>MGSTGNAEIQIIPTHSSDEEANLFAHQLARAASLPMALKAAIELDVLEIMAKSVPPSGYISPAEIAAQLPTTNPEAPVMLDRVLRLLASYSVVTYTLRELPSGKVERLYGLAPVCKFLTKNEDGVSLAPFLLLATDKVLLEPWFYLKDAILEGGIPFNKAYGMNIWDYFGTDHRINKVFNKGMSSNSTITMKKILEMYNGFEGLTTIVDVGGGTGAVASMIVAKYPSINAINFDLPHVIQDAPAFSGVEHLGGDMFDGVPKGDAIFIKWICHDWSDEHCLKLLKNCYAALPDHGKVIVAEYILPPSPDPSIATKV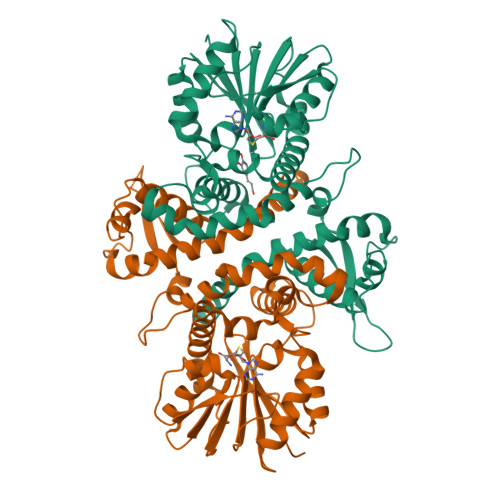VIHMDALMLAYNPGGKERTEKEFQALAMASGFRGFKVASCAFNTYVMEFLKTA[2x]> AMADITSLYKKAESAAAPFTYWLNPEIYDAGGLSRRAFPEGFVFGTAASAYQVEGMAKQGGRGPSIWDAFIEKPGTIPNNATADVTVDEYHRYKEDVNIMKNMGFDAYRFSISWSRIFPNGTGMVNQEGVDYYNRLIDYMVKKGIKPYANLYHYDLPLALHEQYLGWLSPNIVEAFADYADFCFQTFGDRVKDWFTFNEPRCVAALGYDNGFHAPGRCSGCDAGGNSTTEPYLAAHHLILSHAAAVKRYREKYQLYQKGRIGILLDFVWYEPFSDSNADRAAAQRARDFHLGWFLDPIIHGRYPYSMLEIVKDRMPTFSDEESRMVKDSIDYVGINHYTSFYMKDPGPWNLTPTSYQDDWHV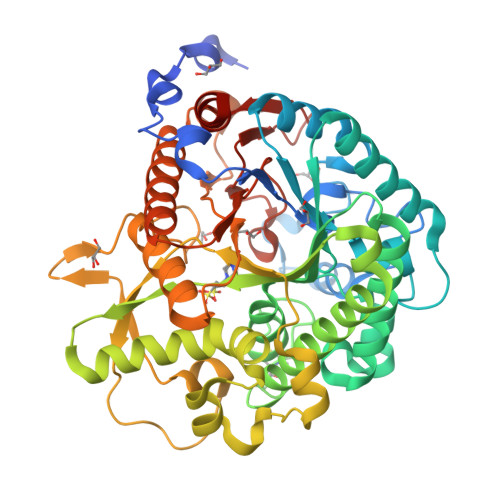GFAYERNGVPIGAQANSYWLYIVPWGINKAVTYVKETYGNPTMILSENGMDQPGNVSITQGVHDTVRIRYYRNYITELKKAIDDGAKVIGYFAWSLLDNFEWRLGYTSRFGIVYVDYKTLKRYPKDSAFWFKNMLSSKKRN>MVARPKSEDKKQALLEAATQAIAQSGIAASTAVIARNAGVAEGTLFRYFATKDELINTLYLHLKQDLCQSMIMELDRSITDAKMMTRFIWNSYISWGLNHPARHRAIRQLAVSEKLTKETEQRADDMFPELRDLCHRSVLMVFMSDE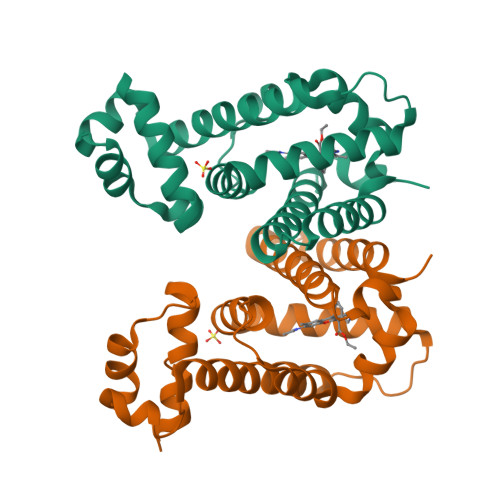YRAFGDGLFLALAETTMDFAARDPARAGEYIALGFEAMWRALTREEQ[4x]>GLIYGNYLHLEKVLNAQELQSETKGNKIHDEHLFIITHQAYELWFKQILWELDSVREIFQNGHVRDERNMLKVVSRMHRVSVILKLLVQQFSILETMTALDFNDFREYLSPASGFQSLQFRLLENKIGVLQNMRVPYNRRHYRDNFKGEENELLLKSEQEKTLLELVEAWLERTPGLEPHGFNFWGKLEKNITRGLEEEFIRIQAKEESEEKEEQVAEFQKQKEVLLSLFDEKRHEHLLSKGERRLSYRALQGALMIYFYREEPRFQVPFQLLTSLMDIDSLMTKWRYNHVCMVHRMLGSKAGTGGSSGYHYLRSTVSDRYKVFVDLFNLSTYLIPRHW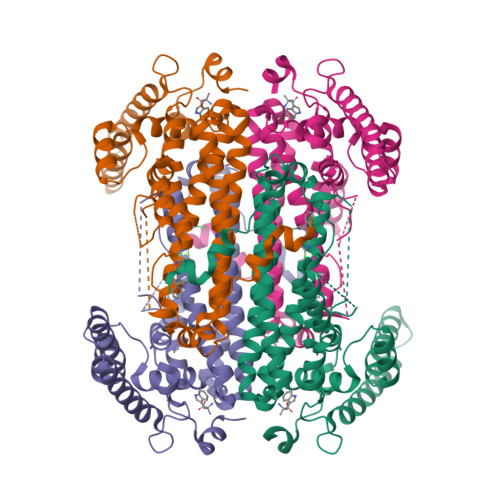IPKMNPTIHKFLEHHHHHH[4x]> PGSLNPCIEVVPNITYQCMDQKLSKVPDDIPSSTKNIDLSFNPLKILKSYSFSNFSELQWLDLSRCEIETIEDKAWHGLHHLSNLILTGNPIQSFSPGSFSGLTSL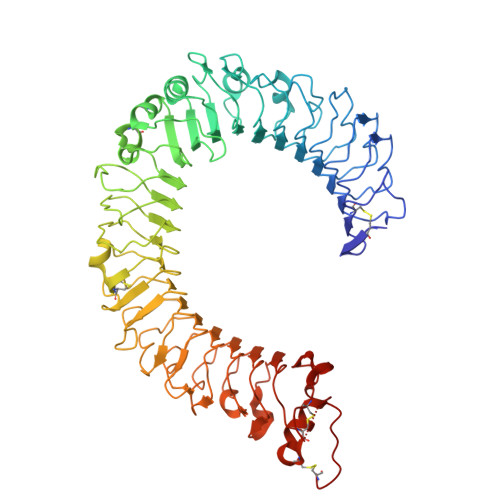ENLVAVETKLASLESFPIGQLITLKKLNVAHNFIHSCKLPAYFSNLTNLVHVDLSYNYIQTITVNDLQFLRENPQVNLSLDMSLNPIDFIQDQAFQGIKLHELTLRGNFNSSNIMKTCLQNLAGLHVHRLILGEFKDERNLEIFEPSIMEGLCDVTIDEFRLTYTNDFSDDIVKFHCLANVSAMSLAGVSIKYLEDVPKHFKWQSLSIIRCQLKQFPTLDLPFLKSLTLTMNKGSISFKKVALPSLSYLDLSRNALSFSGCCSYSDLGTNSLRHLDLSFNGAIIMSANFMGLEELQHLDFQHSTLKRVTEFSAFLSLEKLLYLDISYTNTKIDFDGIFLGLTSLNTLKMAGNSFKDNTLSNVFANTTNLTFLDLSKCQLEQISWGVFDTLHRLQLLNMSHNNLLFLDSSHYNQLYSLSTLDCSFNRIETSKGILQHFPKSLAFFNLTNNSVACICEHQKFLQWVKEQKQFLVNVEQMTCATPVEMNTSLVLDFNNSTCYM>MPFEWVKQYDYEDIIYETYNGIAKITINRPEVHNAFRPKTVNEMIDAFTKARDDSNIGVIILTGAGGKAFCSGGDQKVRGHGGYVGEDEIPRLNVLDLQRLIRVIPKPVIAMVAGYAIGGGHVLHVVCDLTIAADNAIFGQTGPKVGSFDGGYGAGYLARIVGHKKAREIWYLCRQYTAQEALEMGLVNKVVP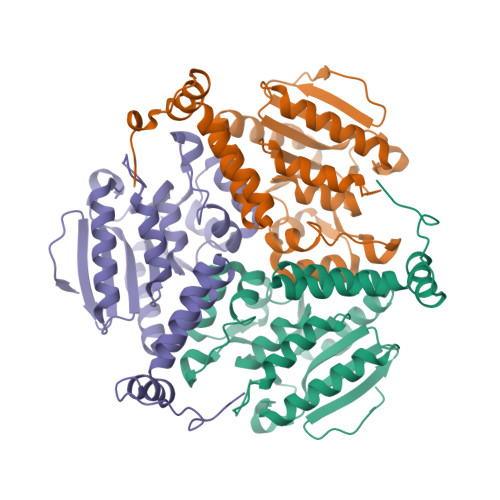LEQLEEETVKWAQEILEKSPTAIRFLKAAFNADSDGLAGIQQLAGDATLLFYTTEEAKEGMRAFKEKRKPDFSQFPRFP[3x]> SKTRQTFSWVGRP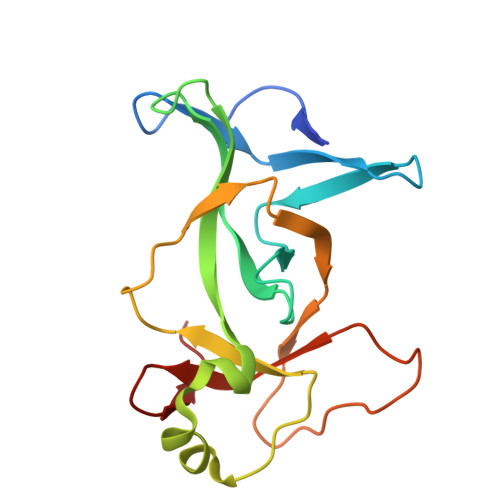LPNRKQFQQMYREICMKINDGSEIHIKVGQFVLIQGEDNKKPYVAKLIELFQNGAEVPPKKCARVQWFVRFLEIPVSKRHLLGRSPPAQEIFWYDCSDWDNKINVETIIGPVQVVALAPEEVIPVDQKSEETLFVKLSWNKKDFAPLPPE>MSLATPHINAQMGDFADVVLMPGDPLRAKYI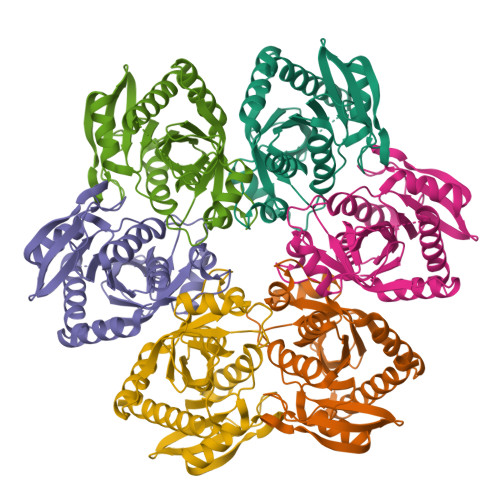AENFLDNAVQVCDVRNMFGYTGTYKGRRISVMGHGMGIPSCSIYVTELIKDYGVKKIIRVGSCGAVNEGIKVRDVVIGMGACTDSKVNRIRFKDHDFAAIADYKMVKAAEEAAKARGIDVKVGNLFSAELFYTPDPSMFDVMDKYGIVGVEMEAAGIYGVAAEYGAKALAICTVSDHIKTGEQTTSEERQNTFNEMIEIALDSVLIGDQAGYEGGSHHHHHH[6x]>[2x]MENFPTEYFLNTTVRLLEYIRYRDSNYTREERIENLHYAYNKAAHHFAQPRQQQLLKVDPKRLQASLQTIVGMVVYSWAKVSKECMADLSIH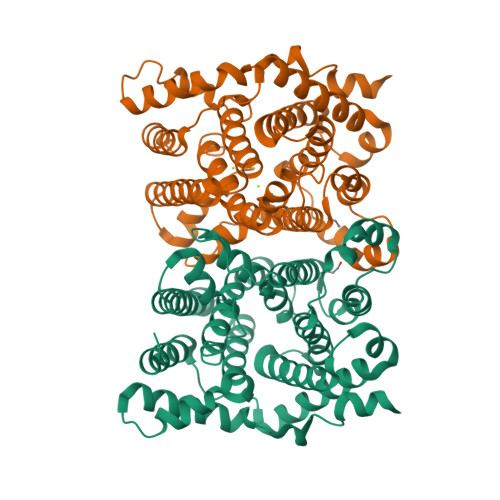YTYTLVLDDSKDDPYPTMVNYFDDLQAGREQAHPWWALVNEHFPNVLRHFGPFCSLNLIRSTLDFFEGCWIEQYNFGGFPGSHDYPQFLRRMNGLGHCVGASLWPKEQFNERSLFLEITSAIAQMENWMVWVNDLMSFYKEFDDERDQISLVKNYVVSDEISLHEALEKLTQDTLHSSKQMVAVFSDKDPQVMDTIECFMHGYVTWHLCDRRYRLSEIYEKVKEEKTEDAQKFCKFYEQAANVGAVSPSEWAYPPVAQLANVRSKDVKEVQKPFLSSIELVE>[2x]MAQILPIRFQEHLQLQNLGINPANIGFSTLTMESDKFICIREKVGEQAQVVIIDMNDPSNPIRRPISADSAIMNPASKVIALKAGKTLQIFNIEMKSKMKAHTMTDDVTFWKWISLNTVALVTDNAVYHWSMEGESQPVKMFDRHSSLAGCQIINYRTDAKQKWLLLTGISAQQNRVVGAMQLYSVDRKVSQPIEGHAASFAQFKMEGNAEESTLFCFAVRGQAGGKLHIIEVGTPPTGNQ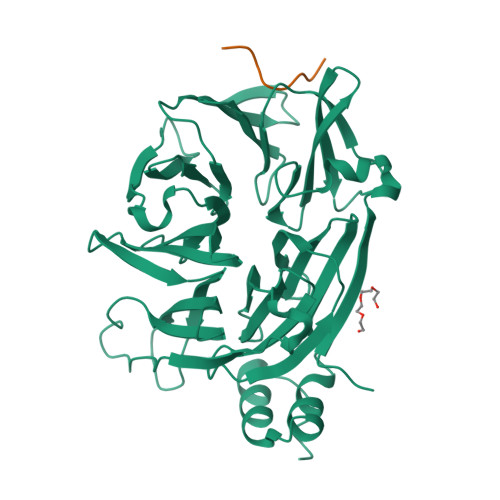PFPKKAVDVFFPPEAQNDFPVAMQISEKHDVVFLITKYGYIHLYDLETGTCIYMNRISGETIFVTAPHEATAGIIGVNRKGQVLSVCVEEENIIPYITNVLQNPDLALRMAVRNNLAGAEELF;>VDGAADLIDFSVPTDEY[2x]>SGEGQDIWDMLDKGNPFQFYLTRVSGVKPKYNSGALHIKDILSPLFGTLVSSAQFNYCFDVDWLVKQYPPEFRKKPILLVHGDKREAKAHLHAQAKPYENISLCQAKLDIAFGTHHTKMMLLLYEEGLRVVIHTSNLIHADWHQKTQGIWLSPLYPRIADGTHKSGESPTHFKADLISYLMAYNAPSLKEWIDVIHKHDLSETNVYLIGSTPGRFQGSQKDNWGHFRLKKLLKDHASSMPNAESWPVVGQFSSVGSLGA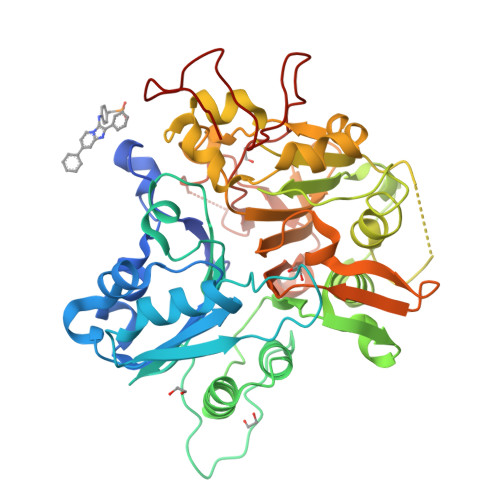DESKWLCSEFKESMLTLGKESKTPGKSSVPLYLIYPSVENVRTSLEGYPAGGSLPYSIQTAEKQNWLHSYFHKWSAETSGRSNAMPHIKTYMRPSPDFSKIAWFLVTSANLSKAAWGALEKNGTQLMIRSYELGVLFLPSAFGLDSFKVKQKFFAGSQEPMATFPVPYDLPPELYGSKDRPWIWNIPYVKAPDTHGNMWVPS[2x]(4-BROMOPHENYL)[4-({(2E)-4-[CYCLOPROPYL(METHYL)AMINO]BUT-2-ENYL}OXY)PHENYL]METHANONE 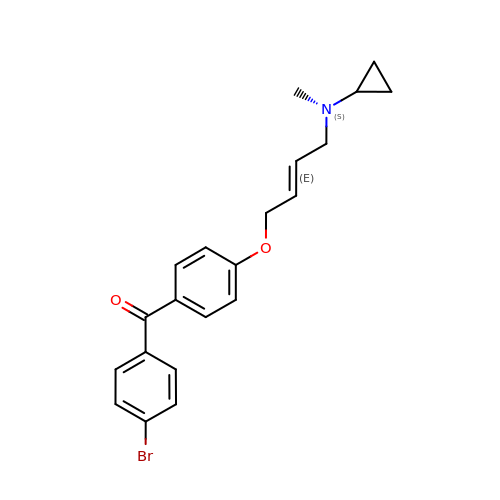| C21 H22 Br N O2 | JAZMZJDLZUDIDG-NSCUHMNNSA-N Cyclophilins are peptidyl-prolyl isomerases (PPIases: EC 5.2.1.8) and are characterized by their ability to catalyze the interconversion of cis and trans isomers of proline. In order to understand the molecular basis of these results, we sought structural coverage of the entire human cyclophilin enzymatic class. We determined crystal structures of seven human PPIase domains—PPIC, PPIE, PPIG, PPWD1, PPIL2, NKTR, and SDCCAG-10 (Figure 2 and Datapack S1). All cyclophilins share a common fold architecture consisting of eight antiparallel β sheets and two α-helices that pack against the sheets. The active site of the cyclophilin family includes the invariant catalytic arginine (Arg55) and a highly conserved mixture of hydrophobic, aromatic, and polar residues including Phe60, Met61, Gln63, Ala101, Phe113, Trp121, Leu122, and His126.

In addition, binding of CsA or derivatives was seen for PPIF, PPIG, PPIH, and NKTR. Modeling of either CsA into the active site of a histidine containing isoform (like NKTR) or computational mutation of the Trp121 in a PPIA∶CsA complex structure indicated that similar hydrogen bond distances can exist between the indole moiety of tryptophan or the imidazole ring of histidine and the carbonyl of methylleucine 9 (MLE9) in CsA. Therefore either residue would be competent for binding, as we have shown experimentally. Conversely, a tyrosine modeled in the conformation to coordinate with CsA created a steric clash with the carbonyl of MLE9 (1.75 Å); in addition, there was a close steric conflict with the modeled Tyr residue and Cζ of the highly conserved Phe60 residue that helps form the proline-binding pocket. Consistent with this, electron density for Phe71 residue in NKTR indicated that alternative conformations are possible for this residue, which may also explain why the PPIA Trp121Tyr mutant was still capable of coordinating substrate in vitro. For instance, the residue that is at position 103 in PPIA varies from alanine in about half of the cyclophilin isoforms to a serine in PPIE, PPIH, and PPIL2; an arginine in PPIG and NKTR; lysine in PPIL6; asparagine in PPIL3 and PPIL4; and glutamine in RANBP2. The occluded set consists of the cyclophilin isoforms with bulky sidechains at the gatekeeper positions; for instance, NKTR has Lys84, Tyr93, and Arg114 compared to PPIA residues Thr73, Lys82, and Ala103. Indeed, for NKTR there were relatively few tetrapeptide combinations with both favorable predicted binding energy and penetration into the S2 pocket; this is easily rationalized by the extremely narrow gap between the gatekeeper 1 and gatekeeper 3 regions in the NKTR structure, which occlude the S2 pocket and restrict the types of residues that can stably associate with the pocket without steric or charge clashes.

>[2x]MGSSHHHHHHSSGLVPRGSPQCHFDIEINREPVGRIMFQLFSDICPKTCKNFLCLCSGEKGLGKTTGKKLCYKGSTFHRVVKNFMIQGGDFSEGNGKGGESIYGGYFKDENFILKHDRAFLLSMANRGKHTNGSQFFITTKPAPHLDGVHVVFGLVISGFEVIEQIENLKTDAASRPYADVRVIDCGVLATK>MVRANKRNEALRIESALLNKIAMLGTEKTAEAVGVDKSQISRWKRDWIPKFSMLLAVLEWGVVDDDMARLAR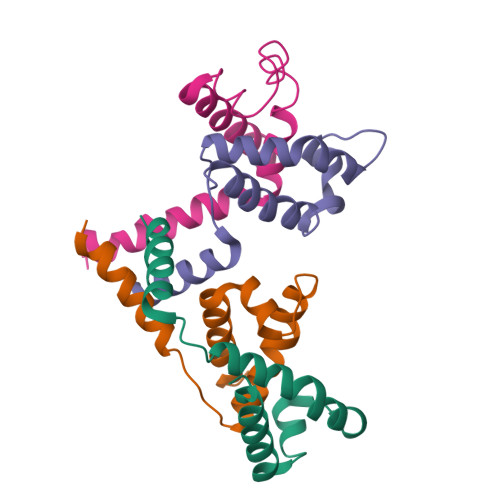QVAAILTNKKRPAATERSEQIQMEF[4x]Influenza A viruses display two membrane-anchored glycoproteins, hemagglutinin (HA) and neuraminidase (NA). After virus replication, NA removes sialic acid residues from viral and cellular glycoproteins to facilitate virus release and allow spread of infection to new cells. NA is a good target for structure-based enzyme inhibitor design because its well-characterized active site is conserved across all influenza A and B viruses. The 11 amino acids in the active site that interact with sialic acid remain unchanged amidst extensive genetic variation in the rest of the sequence; for an alignment, see [9].

We have determined the crystal structure of 2 in complex with a type A N9 NA to a resolution of 1.55 Å, and we discuss it in terms of the successful reorientation of the benzene ring and the lack of improvement in binding affinity. Inhibitor 2 uses benzoic acid to mimic the pyranose ring, a bis-(hydroxymethyl)-substituted 2-pyrrolidinone ring in place of the N-acetyl group of the sialic acid, and a branched aliphatic structure to fill the sialic acid C6 subsite. Structural studies of complexes between several benzoic acid leads and type B NA showed that these inhibitors were bound in the active site in a similar fashion to sialic acid, and the same is observed in the new structure. The carboxylate group of the inhibitor interacts with the guanidinium groups of arginine residues at positions 118, 292, and 371 as seen in all NA substrate and inhibitor complexes and calculated to be energetically important. The pyrrolidine ring interacts with Arg152 by forming a hydrogen bond with its carbonyl oxygen (O15). The one well-ordered propyl chain is anchored by hydrophobic contacts with Ile222, Ala246, and Arg224. The other propyl chain that is disordered is exposed to the solvent and therefore not contributing to binding energy because the one interaction seen is of low occupancy and at the upper limit of the distances considered as significant. The benzene ring of 2 is tilted by 8.9° relative to compound 1, increasing the number of contacts as was predicted in the design. However, one branch of the 3-heptyl group makes no significant contacts due to multiple conformations, which may be why the IC50 is no better than the previous compounds. Most glycans are flexible and only the first few sugars are seen, but the glycan attached to Asn200 is well resolved due to interaction with the adjacent subunit and is seen to contain GlcNAc2Man7.

> IRDFNNLTKGLCTINSWHIYGKDNAVRIGEDSDVLVTREPYVSCDPDECRFYALSQGTTIRGKHSNGTIHDRSQYRALISWPLSSPPTVYNSRVECIGWSSTSCHDGKTRMSICISGPNNNASAVIWYNRRPVTEINTWARNILRTQESECVCHNGVCPVVFTDGSATGPAETRIYYFKEGKILKWEPLAGTAKHIEECSCYGERAEITCTCRDNWQGSNRPVIRIDPVAMTHTSQYICSPVLTDNPRPNDPTVGKCNDPYPGNNNNGVKGFSYLDGVNTWLGRTISIASRSGYEMLKVPNALTDDKSKPTQGQTIVLNTDWSGYSGSFMDYWAEGECYRACFYVELIRGRPKEDKVWWTSNSIVSMCSSTEFLGQWDWPDGAKIEYFL>MATNTDKPVVHYTAPTPNGWVPAILLEELKAVYGGPDYETVKMSIRDADIGKVHNQVKSDWFLKICPNGRIPAITHEGFPVFETSAILLYLAQHFDKENAFSRDPVKDPKGYSEELQWLFFAHGGIGPMQGQANHFNLYAPEKIPYAINRYLNESKRLYRVLDDRLKGREYILGTYGIADIKIFGWARIAPRTGLDLDEFPNVKAWVERIEKRPAVQAG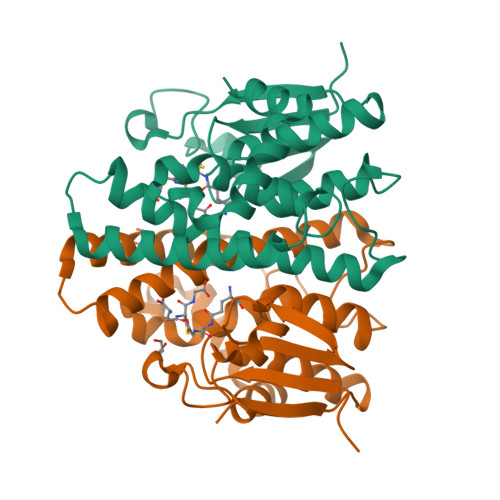INSCN[2x]> GPLG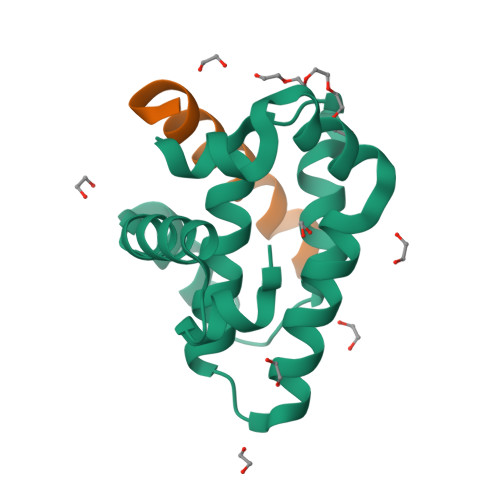SMTNINFSALLRGERMCPLTREIHSQMLIVTKSYSLVETFRAFPRLPNILEIGNNIVSDGNLNWGRILILLGISQLYFTKSESESERTQITEQLERFFRQDAISNWIASNGGWVTCASLDLRNYSSVT;> ALPPEMVVARELRRIGDEFNRLYCEA> SSKIILIPSNIPQEFPEASISNPERLRILAQVKDFIPHESTIVIDKVPTITSEQSTYINICIFNLLEACSSRVLVPGT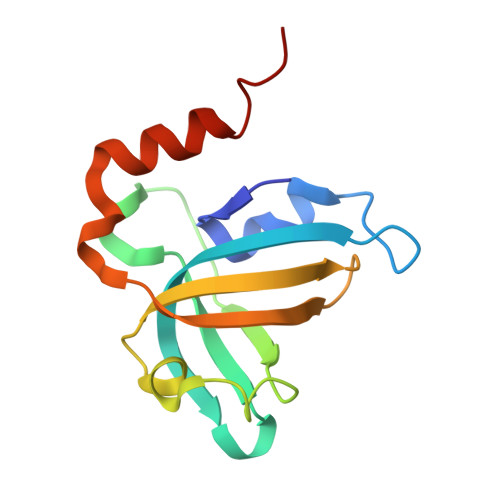LVNIDAFYDGESINPVDIYEVNGANFTMENIQLIDEMNNSIGKFN>[8x]MGLLIDGVWRDAWYDTKSSGGRFVRKESQYRGGLDAGFRGEPGRYHLYAGFACPWAHRVLIMRALKGLEEMISVSMVNAYMGENGWTFLPGDDVVPDSINGADYLYQVYTAADPTYTGRVTIPILWDKVEKRILNNESS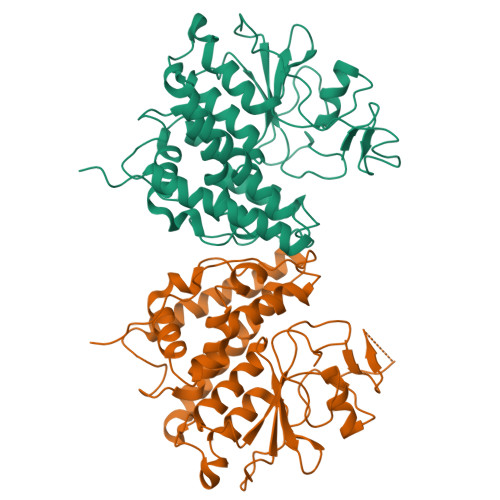EIIRILNSAFDDVGALPGDYYPAEFRPEIDRINARVYETLNNGVYRSGFATTQEAYEEAFYPLFDTLDWLEEHLTGREWLVGDRLTEADIRLFPTLVRFDAIYHGHFKCNLRRIADYPNLSRLVGKLASHERVAPTINLRHAKAHYYGSHPSVNPTGIVPVGPAQPLPGLTLQS>MSYTPGQPVTAVVQRVEIHKLRQGENLILGFSIGGGIDQDPSQNPFSEDKTDKGIYVTRVSEGGPAEIAGLQIGDKIMQVNGWDMTMVTHDQA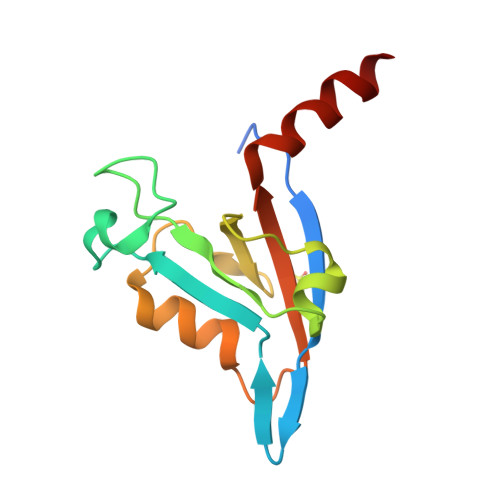RKRLTKRSEEVVRLLVTRQSLQKAVQQSMLS[2x]> MKHHHHHHSAGLEVLFQGP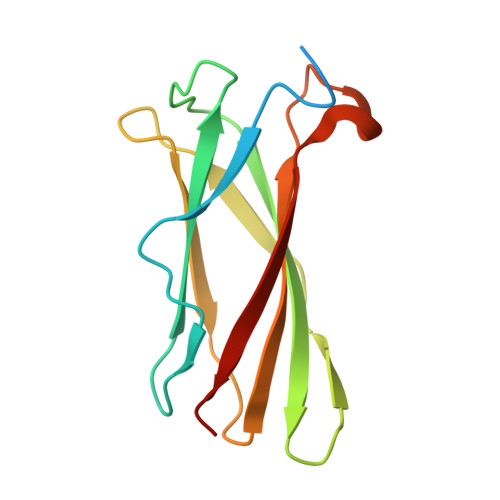MVLSPYKLNLVATPLFLKPGIPYPIKVQVKDSLDQLVGGVPVTLNAQTIDVNQETSDLDPSKSVTRVDDGVASFVLNLPSGVTVLEFNVKTDAPDLPEENQAREGYRAIAYSSL>AKGNDSKDFNNSYGISHITRDNMVKIPQQQNSDQFKVPAFDESTIKNIASAKGKNASGNTIDLDVWDSWPLQNADGTVATYHGYQIVFALAGDPKDSNDTSVYLFYKKAGDKSIDSWKNAGRVFKDSDKFVPNDPHLKNQTQEWSGSGTLTKDGKVRLFYTDYSGKQYGKQTLTTAQVNMSQPNDNTLKVDGVEDYKSIFDGDGKIYQTVQQFIDEGGYDTGDNHTLRDPHYIEDNGHKYLVFEANTGTEDGYQGEDSLYNRAYYGGNNPFFQSEKKKLLEGSNKEKASLANGALGIIELNDDYTLKKVMKPLITSNTVTDEIERANIFKKDGKWYLFT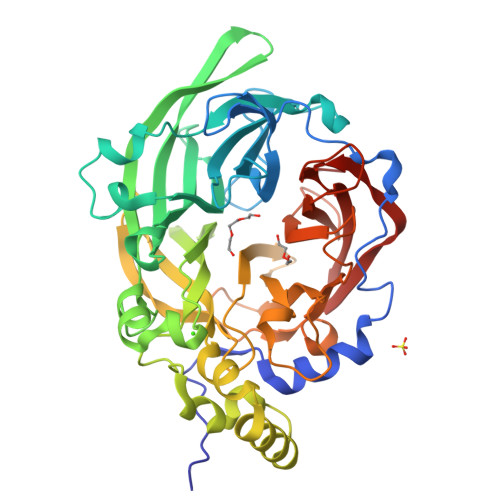DSRGSAMTIDGIGQDDVYMLGYVSNTLTGKYKPLNDTGLVLHMDLDPNDKTFTYSHFAVPQTKGDNVVITSYMTNRGFYEDNHSTFAPSFLVNIDGSKTSVVKDRVLEQGQLTVDED[4x]>[8x]MASQVGAINSVNALISRVFVQPKGDLADRLNSRVTVVILAVSSALLLSSHFIGDPITCWTPAQFNAQWVNFVNQYCFVHGTYFVPLDQQLAFEEEERTKVSIQYYQWVPYVFALQAFLFYIPRFIWKAMIAYSGYDLAAAVKYVDRFWSENRDKDDKFKTRLAAFEGRPSVYIWDGIRLARKKRSRNMALFYTLSTVWQAVNAWIQFYILTQ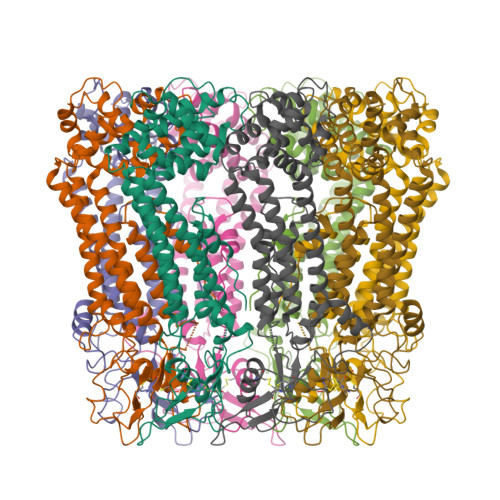LLDSSIYTLWGPSILGDLLQGNDWQTTGHFPRIVHCDFNRRRPASVQLDTVLCVLTLNIYYEKLFIFLWFWLVFVAVVSTVNCFKWIYYLCNKTKAQKTIKNYLSTAPIKSTISDDQFFSALGEDGLFIMDQMALNLGDIPASYLTISMRNICQDFIESEDYIDEERTPFVKSIKHT>MKLSGVELRRVQMPLVAPFRTSFGTQSVRELLLLRAVTPAGEGWGECVTMAGPLYSSEYNDGAEHVLRHYLIPALLAAEDITAAKVTPLLAKFKGHRMAKGALEMAVLDAELRAHERSFAAELGSVRDSVPCGVSVGIMDTIPQLLDVVGGYLDEGYVRIKLKI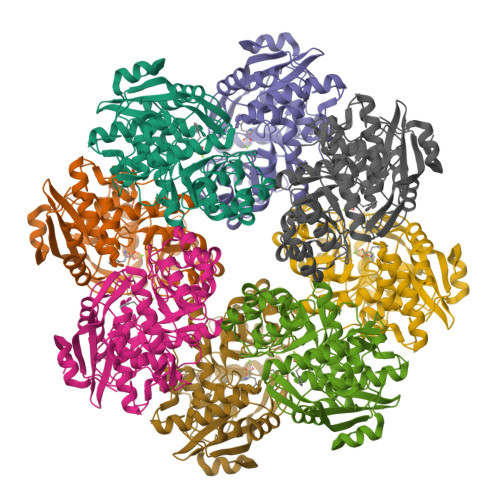EPGWDVEPVRAVRERFGDDVLLQVDANTAYTLGDAPQLARLDPFGLLLIEQPLEEEDVLGHAELARRIQTPICLDESIVSARAAADAIKLGAVQIVNIKPGRVGGYLEARRVHDVCAAHGIPVWCGDMIETGLGRAANVALASLPNFTLPGDTSASDRYYKTDITEPFVLSGGHLPVPTGPGLGVAPIPELLDEVTTAKVWIGS[4x]> GSHMGSPNSPLKDSLRPKLSEEQQHIIAILLDAHHKTYDPTYADFRDFRPP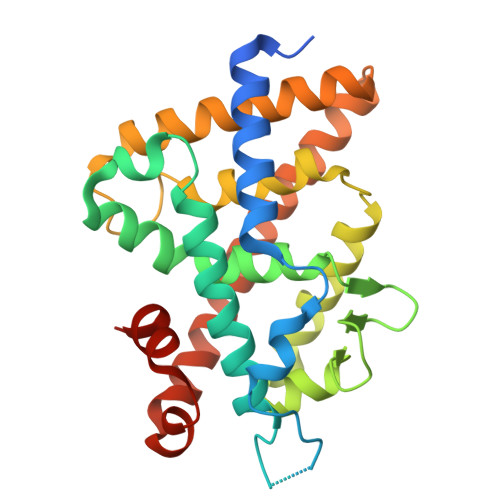VRMDGSTGSVTLDLSPLSMLPHLADLVSYSIQKVIGFAKMIPGFRDLTSDDQIVLLKSSAIEVIMLRSNQSFTMDDMSWDCGSQDYKYDVTDVSKAGHTLELIEPLIKFQVGLKKLNLHEEEHVLLMAICIVSPDRPGVQDAKLVEAIQDRLSNTLQTYIRCRHPPPGSHQLYAKMIQKLADLRSLNEEHSKQYRSLSFQPENSMKLTPLVLEVFGNEIS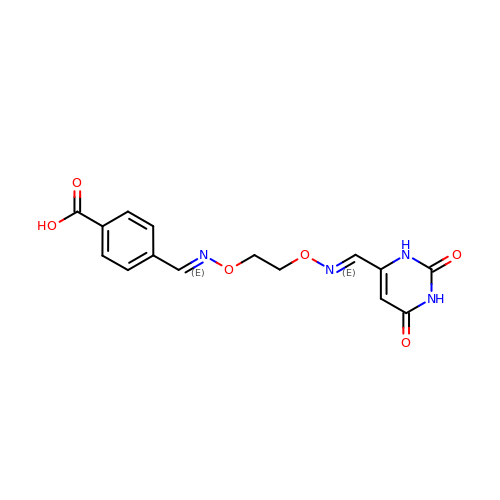4-[(1E,7E)-8-(2,6-DIOXO-1,2,3,6-TETRAHYDROPYRIMIDIN-4-YL)-3,6-DIOXA-2,7-DIAZAOCTA-1,7-DIEN-1-YL]BENZOIC ACID | C15 H14 N4 O6 | XHDKIDMFBWLHAX-GONBZBRSSA-N>LRNATQRMFEIDYSRDSFLKDGQPFRYISGSIHYSRVPRFYWKDRLLKMKMAGLNAIQTYVPWNFHEPWPGQYQFSEDHDVEYFLRLAHELGLLVILRPGPYICAEWEMGGLPAWLLEKESILLRSSDPDYLAAVDKWLGVLLPKMKPLLYQNGGPVITVQVENEYGSYFACDFDYLRFLQKRFRHHLGDDVVLFTTDGAHKTFLKCGALQGLYTTVDFGTGSNITDAFLSQRKCEPKGPLINSEFYTGWLDHWGQPHSTIKTE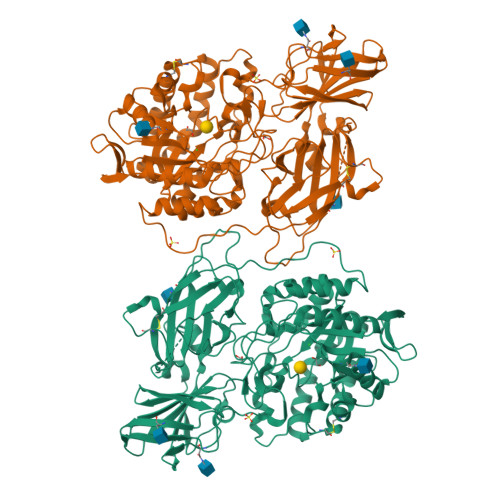AVASSLYDILARGASVNLYMFIGGTNFAYWNGANSPYAAQPTSYDYDAPLSEAGDLTEKYFALRNIIQKFEKVPEGPIPPSTPKFAYGKVTLEKLKTVGAALDILCPSGPIKSLYPLTFIQVKQHYGFVLYRTTLPQDCSNPAPLSSPLNGVHDRAYVAVDGIPQGVLERNNVITLNITGKAGATLDLLVENMGRVNYGAYINDFKGLVSNLTLSSNILTDWTIFPLDTEDAVRSHLGGWGHRDSGHHDEAWAHNSSNYTLPAFYMGNFSIPSGIPDLPQDTFIQFPGWTKGQVWINGFNLGRYWPARGPQLTLFVPQHILMTSAPNTITVLELEWAPCSSDDPELCAVTFVDRPVIGSSVTYDHPSKPVEKRLMPPPPQKNKDSWLDHV[4x]3-HYDROXYPROPYL 3-[({7-[AMINO(IMINO)METHYL]-1-NAPHTHYL}AMINO)CARBONYL]BENZENESULFONATE 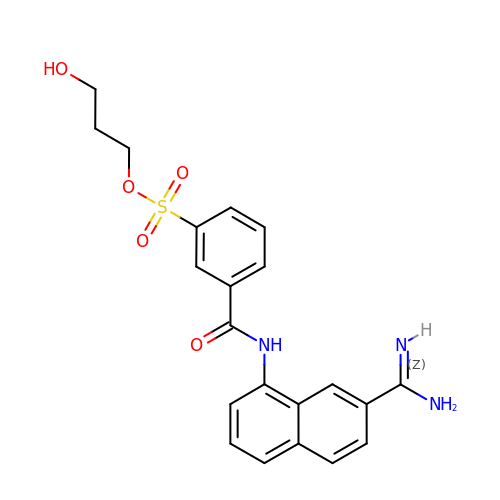| C21 H21 N3 O5 S | PXERBGNIBOFZOW-UHFFFAOYSA-N>HHHHSGDDDDKA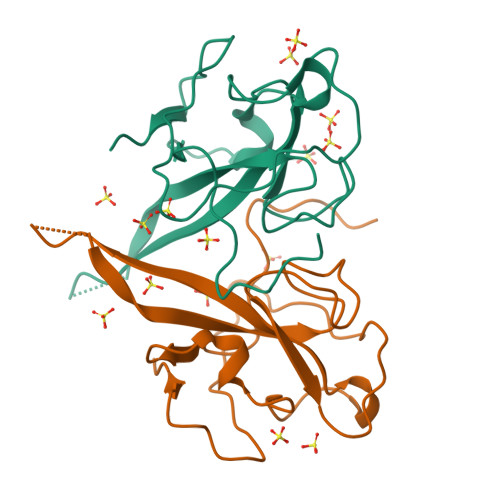SVNWADDRAARKKFPPPSFYMPLLVSSDKAPYRVIPRNLVPIGKGNKDEQIGYWNVQERWRMRRGQRVDLPPKVHFYYLGTGPHKDLKFRQRSDGVVWVAKEGAKTVNTSLGNRKRNQKPLEPKFSIALPPELSVVEF[2x]> GPGSELPQMVQQLNSPDQQELQSALRKLSQIASGGNEQIQAVIDAGALPALVQLLSSPNEQILQEALWALSNIASGGNEQIQAVID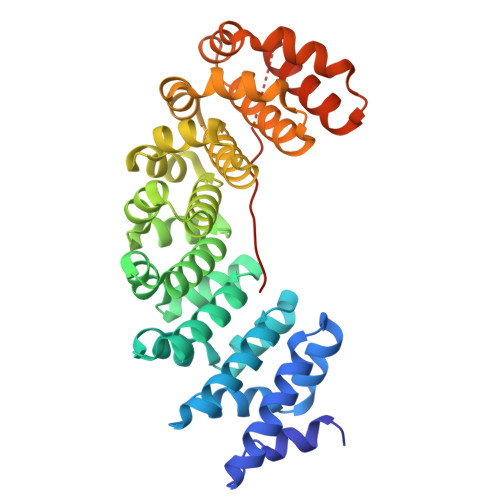AGALPALVQLLSSPNEQILQEALWALSNIASGGNEQIQAVIDAGALPALVQLLSSPNEQILQEALWALSNIASGGNEQIQAVIDAGALPALVQLLSSPNEQILQEALWALSNIASGGNEQIQAVIDAGALPALVQLLSSPNEQILQEALWALSNIASGGNEQIQAVIDAGALPALVQLLSSPNEQILQEALWALSNIASGGNEQKQAVKEAGALEKLEQLQSHENEKIQKEAQEALEKLGGGGSGGGGSGKRKRKRKRKRKRKR> MRGSHHHHHHGSALSNKFIGDDMKMTYHMDGCVNGHYFTVKGEGNGKPYEGTQTSTFKVTMANGGPLAFSFDILSTVFKYGNRCFTAYPTSMPDYFKQAFPDGMSYERTFTYEDGGVATASWEISLKGNCFEHKSTFHGVNFPADGPVMAKKTTGWDPSFEKMTVCDGILKGDVTAFLMLQGGGNYRCQF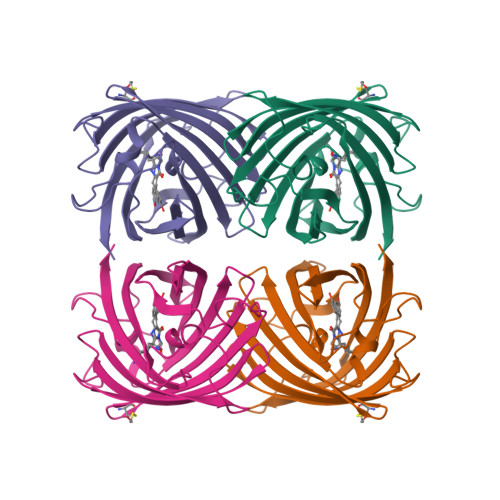HTSYKTKKPVTMPPNHVVETRIARTDLDKGGNSVQLTEHAVAHITSVVPF> MKELNDLEKKYNAHIGVYALDTKSGKEVKFN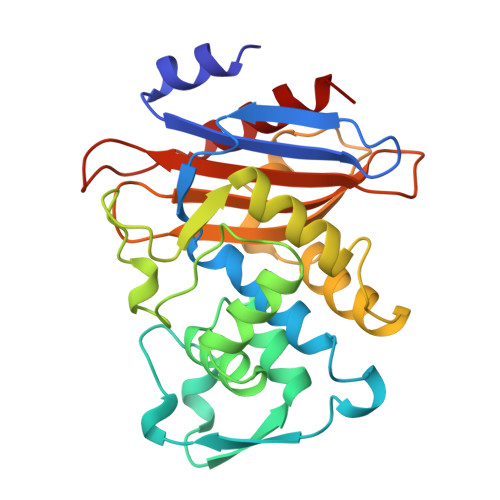SDKRFAYASTSKAINSAILLEQVPYNKLNKKVHINKDDIVAYSPILEKYVGKDITLKALIEASMTYSDNTANNKIIKEIGGIKKVKQRLKELGDKVTNPVRYEIELQYYSPKSKKDTSTPAAFGKTLNKLIANGKLSKENKKFLLDLMLNNKSGDTLIKDGVPKDYKVADKSGQAITYASRNDVAFVYPKGQSEPIVLVIFTNKDNKSDKPNDKLISETAKSVMKEF>MRGSHHHHHHGRSLNPLSTPQFDSTDETPASYNLAVRRAAPAVVNVYNRGLNTNSHNQLEIRTLGSGVIMDQRGYIITNKHVINDADQIIVALQDGRVFEALLVGSDSLTDLAVLKINATGGLPTIPINARRVPHIGDVVLAIGNPYNLGQTITQGIISATGRIGLNPTGRQNFLQTDASINPGNSGGALVNSLGELMGINTLSFDKSNDGETPEGIGFAIPFQLATKIMDKLIRDGRVIRGYIGIGGREIAPLHAQGGGIDQLQGIVVNEVSPDGPAANAGIQVNDLIISVDNKPAI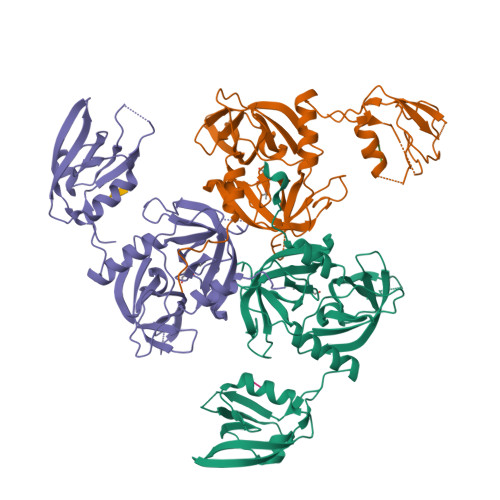SALETMAQVAEIRPGSVIPVVVMRDDKQLTLQVTIQEYPATN[3x];>[3x]YQF> GNSVTNIYGNGNNVTTDVGANGWAPTVSTGLGDGPVSASADSLPGRSGGASSEKTHTVSGSSNKVGSRFSKWWEPAAARASESATDSAIEGIDAAGKAASKAITRKLDRPAAPSSTANPQPSLIALNPSATQSGNASILTGSTAPSLLAYPTATPVP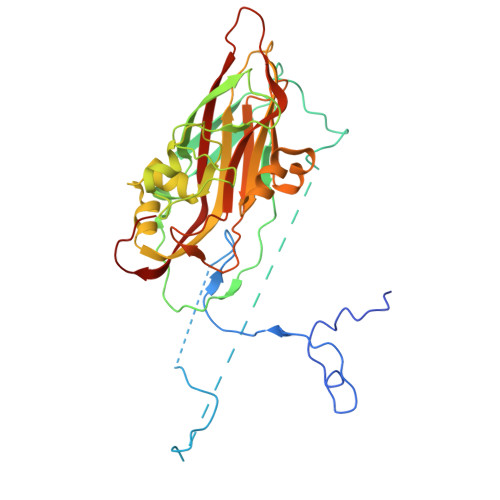LPNPDEPSQPGPSGDRTWLLDTVTWSQEFTRGWNIAGSNGMQWTGLESLIFPVSTDTNWTSTSSPTAYPLPFSFVRAYPDSSWAAMYNTHSMWNCGWRVQVTVNGSQFHAGALILYMVPEATTHAIQTARDNAGFVFPYVILNLYESNTATIEVPYISPTPNTSSGLHAPWTFYLQVLSPLNPPPSLPTSLSCSIYVTPVDSSFHGLRYLAPQ>[6x]GSSERPSPPVNLTSSDQTQSSVQLKWEPPLKDGGSPILGYIIERCEEGKDNWIHCNMKLVPELTYKVTGLEKGNKYLYRVSAENKAGVSDPSEILGPLTADDAFVE

Titin is a protein expressed in the skeletal and cardiac, or striated, muscle of vertebrates that plays various roles in muscle structure and function. Encoded by the gene TTN, titin spans half a sarcomere (the basic contractile unit of muscle) and has various functions including preventing sarcomere over-extension (Gautel and Djinović-Carugo, 2016), acting as a molecular ruler for thick filament formation and as a hub for numerous signalling molecules (Kruger and Linke, 2011, Linke and Hamdani, 2014). Fn3 domains are only found in the A-band region of titin, where they are arranged with Ig domains in a pattern termed super-repeats, which themselves are repeated. Fn3 domains have a characteristic beta sandwich fold, with a core of hydrophobic residues as the “filling” between two beta sheets that pack against each other face-to-face.

Here, we present the crystal structures of seven human WT titin domains – Fn3-3, Fn3-11, Fn3-20, Fn3-49, Fn3-56, Fn3-85 and Fn3-90 – and two domains harbouring rare missense variants found in patients with HCM: Fn3-3 Arg15908His and Fn3-56 Ser23226Gly. In addition to the WT domains, the structures of Fn3-3 Arg15908His and Fn3-56 Ser23226Gly were determined to a resolution of 2.10 and 1.43 Å, respectively. The two rare missense variants have each been identified in 12 patients of an 874-patient HCM cohort at UCLH, with general population minor allele frequencies (MAFs) of 6.5 × 10-3 and 7.2 × 10-3 for Arg15908His and Ser23226Gly, respectively, suggesting they may play a role in the patients’ disease. There is usually a positively charged residue at the Arg15908 domain position, and the Ser23226 position is also highly conserved. The two variant domains, which each harbour a rare missense variant found in a cohort of HCM patients, closely align with their respective WT domains, with the mutated residue incorporated into the domain without affecting its conformation. Both the Arg15908His variant in Fn3-3, and Ser23226Gly variant in Fn3-56, however, result in the loss of polar contacts, and this is reflected in the loss of thermal stability of the domains. The other four variants were folded so we compared the thermal stability of these WT and variant domains using differential scanning fluorimetry. The melting temperatures, Tm, are shown in Table 2; briefly, the WT domains had Tms of between 59.8 and 74.3 °C and the variant domains had Tms between 46.8 and 66.9 °C, with a reduction in thermal stability ranging from 7.4 °C for Fn3-3 Arg15908His to 13.0 °C for Fn3-90 Arg27839Gln. The high melting temperatures for two of the variant domains (66.9 °C for Fn3-3 Arg15908His and 53.4 °C for Fn3-56 Ser23226Gly) suggest that for these it is the former, as previously characterized variants linked to disease via domain instability typically reduce the domain melting temperature to below physiological levels.> GSMDALNSKEQQEFQKVVEQKQMKDFMRLYSNLVERCFTDCVNDFTTSKLTNKEQTCIMKCSEKFLKHSERVGQRFQEQNAALGQGLGR;> GSMSFLGFGGGQPQ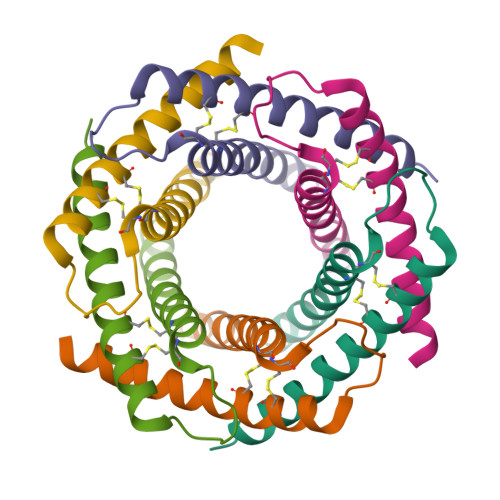LSSQQKIQAAEAELDLVTDMFNKLVNNCYKKCINTSYSEGELNKNESSCLDRCVAKYFETNVQVGENMQKMGQSFNAAGKF> MSDITKIKQEFDKKVAEIQAL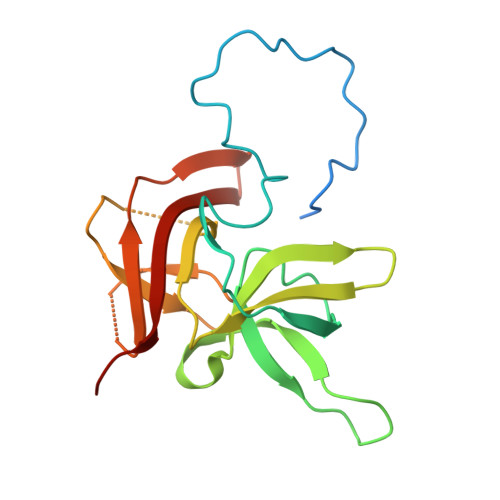MKNPQQDSGLLSNSIDFRDQNLIFSNSGGVCTSSKDKIENYPAKGYPYKRGVKLSFGDGTTELEVEAGGGDDLYGVCSDIDEFSGMATVIPITNNFTGYLTLKKDGQNGVNPGDKLNFNQHGELEKVTGAQKSVNAIALSKAHKLTEDLFIVLASVFGNRAIKG>[2x]MELRVGNRYRLGRKIGSGSFGDIYLGTDIAAGEEVAIKLECVKTKHPQLHIESKIYKMMQGGVGIPTIRWCGAEGDYNVMVMELLGPSLEDLFNFCSRKFSLKTVLLLADQMISRIEYIHSKNFI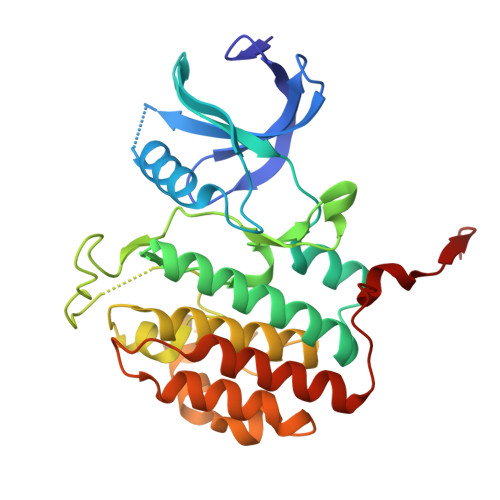HRDVKPDNFLMGLGKKGNLVYIIDFGLAKKYRDARTHQHIPYRENKNLTGTARYASINTHLGIEQSRRDDLESLGYVLMYFNLGSLPWQGLKAATKRQKYERISEKKMSTPIEVLCKGYPSEFATYLNFCRSLRFDDKPDYSYLRQLFRNLFHRQGFSYDYVFDWNMLKFGASR>[4x]GSHMESRALPADEEASAFRAVADPTR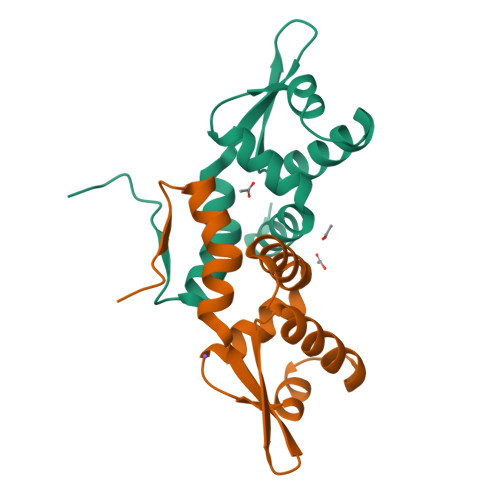RQILEDLRGGELAAGEIAGRFPISAPSISRHLGVLKGAGLVTERRDANRILYSLAEERLALCVGRFLSAVCPEQIVLRTTKWRSAPEGDAS>GSLHMSFETRFEKMDNLLRDPKSEVNSDCLLDGLDALVYDLDFPALRKNKNIDNFLSRYKDTINKIRDLR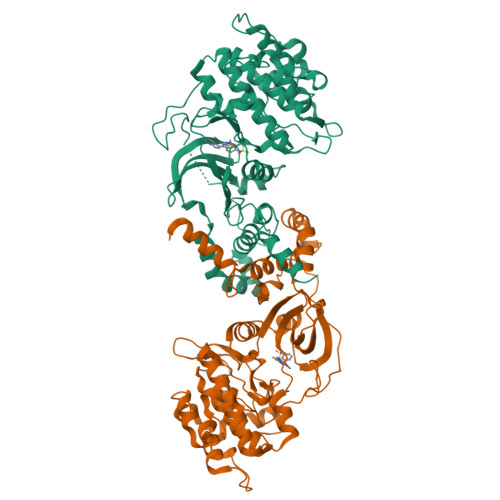MKAEDYEVVKVIGRGAFGEVQLVRHKSTRKVYAMKLLSKFEMIKRSDSAFFWEERDIMAFANSPWVVQLFYAFQDDRYLYMVMEYMPGGDLVNLMSNYDVPEKWARFYTAEVVLALDAIHSMGFIHRDVKPDNMLLDKSGHLKLADFGTCMKMNKEGMVRCDTAVGTPDYISPEVLKSQGGDGYYGRECDWWSVGVFLYEMLVGDTPFYADSLVGTYSKIMNHKNSLTFPDDNDISKEAKNLICAFLTDREVRLGRNGVEEIKRHLFFKNDQWAWETLRDTVAPVVPDLSSDIDTSNFDDLEEDKGEEETFPIPKAFVGNQLPFVGFTYYSNRRYLSSANPNDNR[2x]> MLPLSIEQRRPSRSPEYDQSTLSNYKDFAVLHTDLNLSVSFEKSAISGSVTFQLKKLHEGKNKSDELHLDTSYLDVQEVHIDGSKADFQIEQRKEPLGSRLVINNASCNDNFTLNIQFRTTDKCTALQWLNSKQTKGGKPYVFSQLEAIHARSLFPCFDTPSVKSTFTASIESPLPVVFSGIRIEDTSKDTNIYRFEQKVPIPAYLIGIASGDLSSAPIGPRSTVYTEPFRLKDCQWEFENDVEKFIQTAEKIIFEYEWGTYDILVNVDSYPYGGMESPNMTFATPTLIAHDRSNIDVIAHELAHSWSGNLVTNCSWNHFWLNEGWTVYLERRIIGAIHGEPTRHFSALIGWSDLQNSIDSMKDPERFSTLVQNLNDNTDPDDAFSTVPYEKGFNLLFHLETILGGKAEFDPFIRHYFKKFAKKSLDTFQFLDTLYEFYPEKKEILDSVDWETWLYKPGMPPRPHFITALADNVYQLADKWVEMAQHLKTTEDFRSEFNAIDIKDFNSNQLVLFLETLTQNGHSNKKPKDFDWAKFPVASRALLDIYQDNIVKSQNAEVVFKMF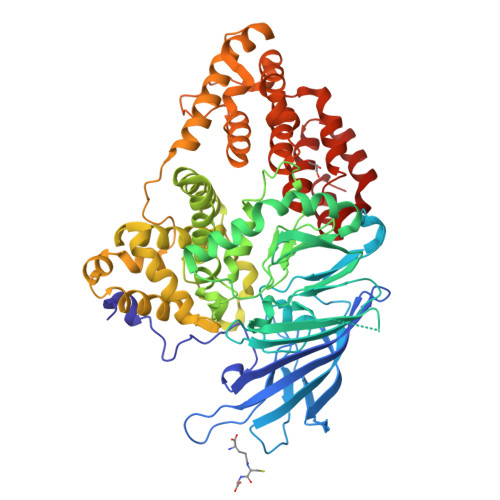KFQIFAKLQEEYKHLADWLGTVGRMKFVRPGYRLLNSVDRRLALATFDKFKDTYHPICKALVKQDLGL> MGNIMSASFAPECTDLKTKYDSCFNEWYSEKFLKGK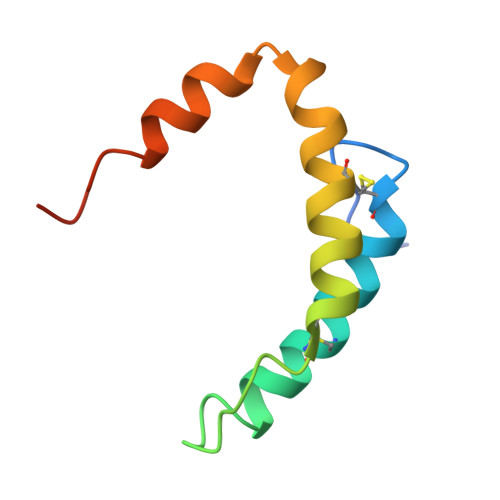SVENECSKQWYAYTTCVNAALVKQGIKPALDEAREEAPFENGGKL Deoxyribose-5-phosphate aldolases (DERAs) are acetaldehyde-dependent, Class I aldolases catalysing in nature a reversible aldol reaction between an acetaldehyde donor (C2 compound) and glyceraldehyde-3-phosphate acceptor (C3 compound, C3P) to generate deoxyribose-5-phosphate, DRP (C5 compound). The 3D structures of several DERA enzymes have been solved, and there are also a few complex structures available. These have revealed that despite of relatively low sequence identity, all DERA enzymes have the ubiquitous TIM (α/β)8-barrel fold where the catalytic amino acids as well as other amino acid residues around the active site seem to be relatively well conserved. The DERA reaction proceeds via Schiff base formation between an active site lysine residue (K167 in Ec DERA) and the donor acetaldehyde substrate. The active site of DERA is located in a deep binding cleft, where the donor acetaldehyde binds to the bottom of the cleft and the acceptor glyceraldehyde-3-phosphate to the upper part, near the cleft entrance.

The crystal structures of two variants of Ec DERA were determined, in order to elucidate mutation-induced changes in the 3D protein structure. The crystal structure of Ec DERA N21K variant, which had lowered specific activity on DRP, and wild-type like activity on DR and acetaldehyde, was determined with and without the ligand, D-2-deoxyribose-5-phosphate (DRP). Diffraction resolutions for all three structures were high (1.5 to 1.9 Å) and the crystallographic R-factors were very low, indicative of high quality 3D structures in each case. In addition, in both N21K crystal structures, there are slight (about 0.2 to 0.4 Å) movements in the positions of altogether three active site loops containing residues G171, G204 and L20, respectively, when compared with the wild-type DERA crystal structure. The N21K mutation is located in the third loop. These small movements slightly narrow the access to the active site of the N21K variant and may thus contribute to the decreased activity against DRP in many of the N21K containing double mutants tested in this work.

>[2x]MTDLKASSLRALKLMDLTTLKDDDTDEKVIALCHQAKTPVGNTAAICIYPRFIPIARKTLKEQGTPEIRIATVTNFPHGNDDIDIALAETRAAIAYGADEVDVVFPYRALMAGNEQVGFDLVKACKEACAAANVLLKVIIETGELKDEALIRKASEISIKAGADFIKTSTGKVAVNATPESARIMMEVIRDMGVEKTVGFKPAGGVRTAEDAQKYLAIADELFGADWADARHYRFGASSLLASLLKALGH> MPLAFCGTENHSAAYRVDQGVLNNGCFVDALNVVPHVFLLFITFPILFIGWGSQSSKVHIHHSTWLHFPGHNLRWILTFILLFVLVCEIAEGILSDGVTESRHLHLYMPAGMAFMAAITSVVYYHNIETSNFPKLLIALLIYWTLAFITKTIKFVKFYDHAIGFSQLRFCLTGLLVILYGMLLLVEVNVIRVRRYIFFKTPREVKPPEDLQDLGVRFLQPFVNLLSKGTYWWMNAFIKTAHKKPIDLRAIGKLPIAMRALTNYQRLCVAFDAQARKDTQSPQGARAIWRALCHAFGRRLILSSTFRILADLLGFAGPLCIFGIVDHLGKENHVFQPKTQFLGVYFVSSQEFLGNAYVLAVLLFLALLLQRTFLQASYYVAIETGINLRGAIQTKIYNKIMHLSTSNLSMGEMTAGQICNLVAIDTNQLMWFFFLCPNLWAMPVQIIVGVILLYYILGVSALIGAAVIILLAPVQYFVATKLSQAQRSTLEHSNERLKQTNEMLRGMKLLKLYAWESIFCSRVEVTRRKEMTSLRAFAVYTSISIFMNTAIPIAAVLITFVGHVSFFKESDLSPSVAFASLSLFHILVTPLFLLSSVVRSTVKALVSVQKLSEFLSSAEIREEQCAPREPAPQGQAGKYQAVPLKVVNRKRPAREEVRDLLGPLQRLAPSMDGDADNFCVQIIGGFFTWTPDGIPTLSNITIRIPRGQLTMIVGQVGCGKSSLLLATLGEMQKVSGAVFWNSNLPDSEGEDPSSPERETAAGSDIRSRGPVAYASQKPWLLNATVEENITFESPFNKQRYKMVIEACSLQPDIDILPHGDQTQIGERGINLSGGQRQRISVARALYQQTNVVFLDDPFSALDVHLSDHLMQAGILELLRDDKRTVVLVTHKLQYLPHADWIIAMKDGTIQREGTLKDFQRSECQLFEHWKTLMNRQDQELEKETVMERKASEPSQGLPRAMSSRDGLLLDEEEEEEEAAESEEDDNLSSVLHQRAKIPWRACTKYLSSAGILLLSLLVFSQLLKHMVLVAIDYWLAKWTDSALVLSPAARNCSLSQECDLDQSVYAMVFTLLCSLGIVLCLVTSVTVEWTGLKVAKRLHRSLLNRIILAPMRFFETTPLGSILNRFSSDCNTIDQHIPSTLECLSRSTLLCVSALTVISYVTPVFLVALLPL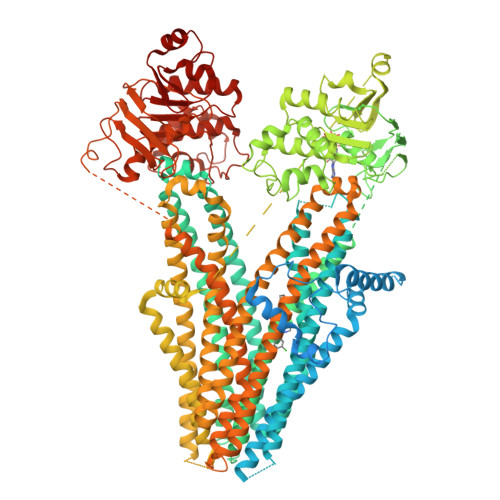AVVCYFIQKYFRVASRDLQQLDDTTQLPLLSHFAETVEGLTTIRAFRYEARFQQKLLEYTDSNNIASLFLTAANRWLEVRMEYIGACVVLIAAATSISNSLHRELSAGLVGLGLTYALMVSNYLNWMVRNLADMEIQLGAVKRIHALLKTEAESYEGLLAPSLIPKNWPDQGKIQIQNLSVRYDSSLKPVLKHVNALISPGQKIGICGRTGSGKSSFSLAFFRMVDMFEGRIIIDGIDIAKLPLHTLRSRLSIILQDPVLFSGTIRFNLDPEKKCSDSTLWEALEIAQLKLVVKALPGGLDAIITEGGENFSQGQRQLFCLARAFVRKTSIFIMDEATASIDMATENILQKVVMTAFADRTVVTIAHRVHTILSADLVMVLKRGAILEFDKPETLLSQKDSVFASFVRADK> 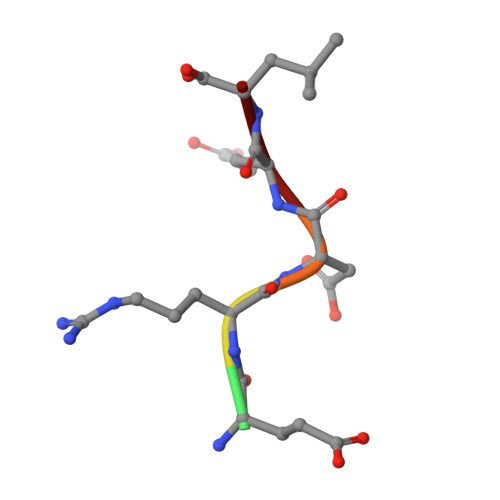AERDEL> MNNTEENIDRIQEPTREDIDRKEAERLLDEAFNPRTKPVDRKKIINSALKILIGLYKEKKDDLTSASFISIARAYYLVSITILPKGTTIPEKKKEALRKGIEFIDRAINKFNGSILDSQRAFRIKSVLSIEFNRIDREKCDNIKLKNLLNEAVDKGCTDFDTYEWDIQIAIRLCELGVDMEGHFDNLIKSNKANDLQKAKAYYFIKKDDHKAKEHMDKCTASLKYTPCSHRLWDETVGFIERLKGDSSTLWRDFAIKTYRSCRVQEKETGTLRLRWYWSRHRVLYDMAFLA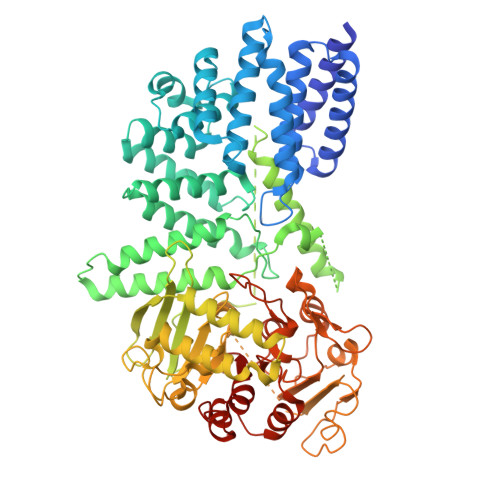VKEQADDEEPDVNVKQAKIKKLAEISDSLKSRFSLRLSDMEKMPKSDDESNHEFKKFLDKCVTAYQDGYVINRSEDKEGQGENKSTTSKQPEPRPQAKLLELTQVPEGWVVVHFYLNKLEGMGNAIVFDKCANSWQYKEFQYKELFEVFLTWQANYNLYKENAAEHLVTLCKKIGETMPFLFCDNFIPNGKDVLFVPHDFLHRLPLHGSIENKTNGKLFLENHSCCYLPAWSFASEKEASTSDEYVLLKNFDQGHFETLQNNQIWGTQSVKDGASSDDLENIRNNPRLLTILCHGEANMSNPFRSMLKLANGGITYLEILNSVKGLKGSQVILGACETDLVPPLSDVMDEHYSVATALLLIGAAGVVGTMWKVRSNKTKSLIEWKLENIEYKLNEWQKETGGAAYKDHPPTFYRSIAFRSIGFPL>MIIGYARVSSLDQNLERQLENLKTFGAEKIFTEKQ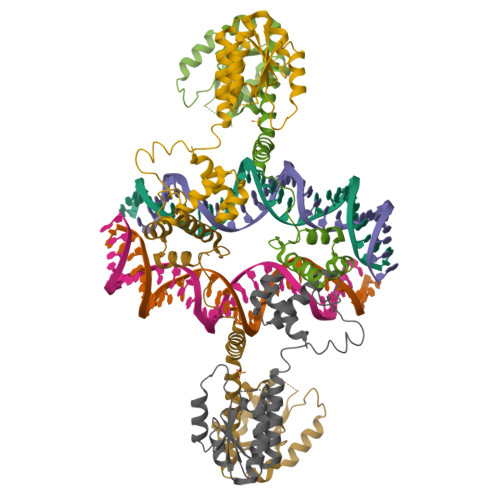SGKSIENRPILQKALNFVRMGDRFIVESIDRLGRNYNEVIHTVNYLKDKEVQLMITSLPMMNEVIGNPLLDKFMKDLIIQILAMVSEQERNESKRRQAQGIQVAKEKGVYKGRPLLYSPNAKDPQKRVIYHRVVEMLEEGQAISKIAKEVNITRQTVYRIKHDNGLSSHHHHHH[4x]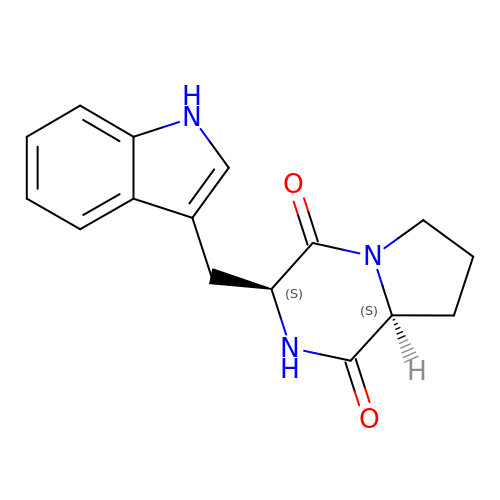(3S,8aS)-3-(1H-indol-3-ylmethyl)hexahydropyrrolo[1,2-a]pyrazine-1,4-dione | C16 H17 N3 O2 | RYFZBPVMVYTEKZ-KBPBESRZSA-N7-amino-N-hydroxyheptanamide | C7 H16 N2 O2 | 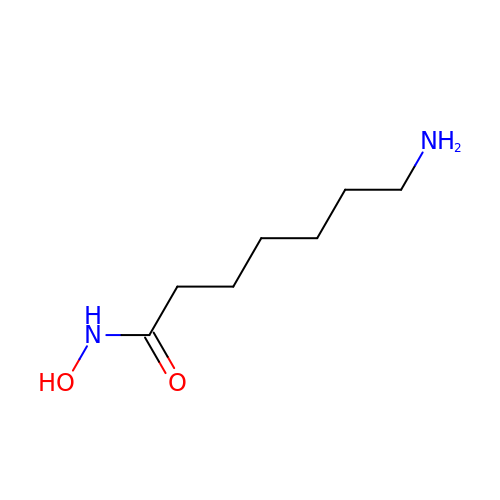ZNRIHNWROBMJQJ-UHFFFAOYSA-N> GPGSNEATASTPVQYWQHHPEKLIFQSCDYKAFYLGSMLIKELRGTESTQDACAKMRANCQKSTEQMKKVPTIILSVSYKGVKFIDAANKNIIAEHEIRNISCAAQDPEDLSTFAYITKDLKSNHHYCHVFTAFDVNLAYEIILTLGQAFEVAYQLAL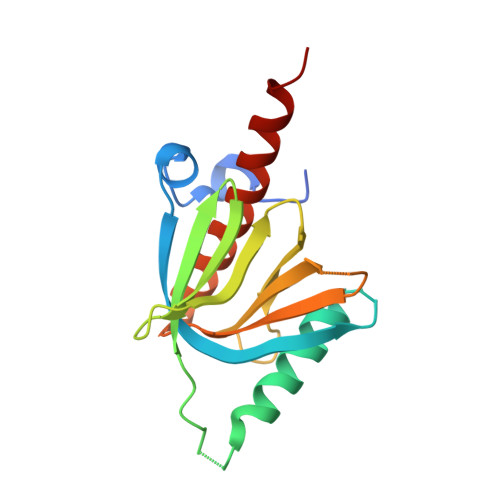QARK>[3x]MHLKIVCLSDEVREMYKNHKTHHEGDSGLDLFI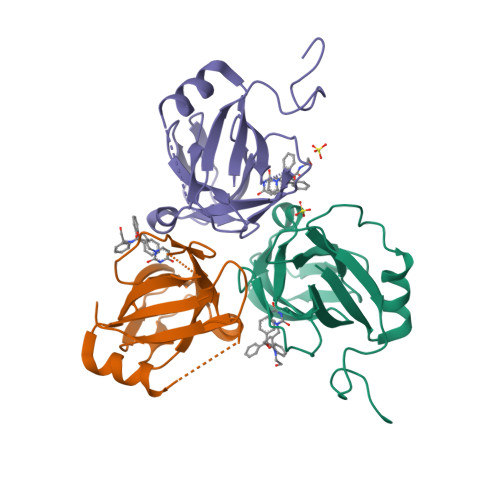VKDEVLKPKSTTFVKLGIKAIALQYKSNYYYKCEKSENKKKDDDKSNIVNTSFLLFPRSSISKTPLRLANSIGLIDAGYRGEIIAALDNTSDQEYHIKKNDKLVQLVSFTGEPLSFELVEELDETSRGEGGFGSTSNNKY> AQVLRGTVTDFPGFDGRADAETLRKAMKGLGTDEESILTLLTSRSNAQRQEISAAFKTLFGRDLLDDLKSELTGKFEKLIVALMKPSRLYDAYELKHALKGAGTNEKVLTEIIASRTPEELRAIKQVYEEEYGSSLEDDVVGDTSGYYQRMLVVLLQANRDPDAGIDEAQVEQDAQALFQAGELKWGTDEEKFITIFGTRSVSHLRKVFDKYMTISGFQIEETIDRETSGNLEQLLLAVVKSIRSIPAYLAETLYYAMKGAGTDDHTLIRVMVSRSEIDLFNIRKEFRKNFA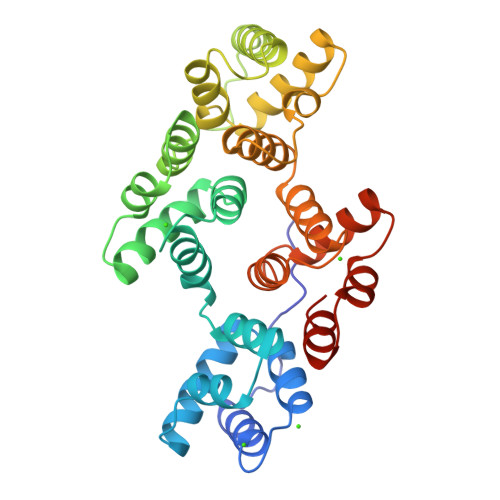TSLYSMIKGDTSGDYKKALLLLCGEDD>[3x]AMKIGVIGAGTMGQGIAKAFAQVEGNTVALCDIKQEWAENGLAKIKKGYEKLVAKGKIPQEKADAIVAAITPGLKENLCADCDLIVEAAFEDMKVKQTTFGELDKICKPECIFASNTASLSITEIGKGLSRPLVGMHFFNPADRMKLIEVIAGCNTPAETVEKIKEISVAIGKNPVQVNEAAGFVVNRILIPMINEAAFIKMEGVSDIAGIDTAMKLGANHPMGPLELGDFIGLDICLAIMDVLYHETGDSKYRACPLIRKMVRGGNLGCKTGKGFYVYNADRTKTPVDN

The A2HBD has elevated expression in F. prausnitzii A2-165 and is crucial for the transformation of acetoacetyl-CoA to 3-hydroxybutyryl-CoA in the butyrate cycle. The monomeric structure of A2HBD consists of two domains, N-terminal and C-terminal, with cofactor binding occurring at the N-terminal domain, while the C-terminal domain facilitates dimerization. The A2HBD protein exists as a hexamer in solution.

Additionally, X-ray data of A2HBD in complex with acetoacetyl-CoA at a resolution of 1.9 Å were collected at PAL-XFEL (fourth generation) utilizing Serial Femtosecond Crystallography (SFX). Due to the limited resolution of the electron density map in the adenine moiety of acetoacetyl-CoA obtained from the tertiary structure analysis, a detailed examination of the binding mode between the adenine moiety of the substrate and the enzyme was conducted using fourth-generation PAL-XFEL diffraction data. The structures formed almost the same conformation with the RMSD of 0.19Å. Arg143 (NH1) forms a hydrogen bond with O30 of the substrate within a 3.00 Å distance. The guanidinium moiety is oriented towards the aromatic ring of the adenine moiety in a stacked (parallel) configuration, with a proximate distance (below 4 Å) between the guanidinium and adenine planes. This arrangement suggests the formation of a cation-π interaction that contributes to the substrate′s stabilization. Notably, residue R143 plays a critical role in capturing the adenine phosphate ring, underlining its significance in substrate recognition and catalytic activity.However, one distinctive member of the YkuD-type transpeptidase family, LdtF (recently renamed DpaA), carries out the opposite reaction of detaching Lpp from the peptidoglycan layer. DpaA specifically hydrolyzes the amide bond between mDAP in PG and the C-terminal L-lysine of Lpp, in a reaction that is the opposite of the Lpp attachment reactions catalyzed by some of the Ldt enzymes. In this study, we report the crystal structure of DpaA, which reveals the enzyme’s ability to cleave, rather than form, the Lpp-peptidoglycan linkage. Assays with purified peptidoglycan-Lpp as the substrate and chemically synthesized compounds suggest that DpaA’s shallow L-shaped active site can only accommodate and cleave the peptidoglycan-Lpp cross-link with a constrained conformation.

However, by treating purified sDpaA with V8 protease, we were able to obtain crystals of the V8-trimmed wild-type sDpaA. Subsequently, we collected a 2.9 Å resolution data set using synchrotron radiation. sDpaA forms a pseudosymmetric dimer in the crystal structure. The final model for both chains A and B in the asymmetric unit includes residues 36-229 and 36-224, respectively. Unlike other YkuD family members, DpaA is a compact protein of a single domain composed of a single mixed five-stranded β-sheet (β1-3 and β4-5), which is flanked by four α-helices and one pair of β-strands (β6-7). Unlike other YkuD-like transpeptidases, sDpaA’s second mixed β-sheet region (Val98-Ala145) is degenerated and instead consists of five coiled strands that are connected by only a few backbone hydrogen bonds. The catalytic Cys143 residue is located in a sharp elbow turn of the coils and is surrounded by three loops (L1–3). These loops create a shallow substrate-binding groove. Our study has revealed that DpaA forms a shallow substrate-binding cleft, with the catalytic Cys143 accessible through a single entrance, similar to LD-CPases. By contrast, DpaA and CPases have a shortened L2 loop, resulting in an uncovered substrate-binding site.

>MGLLGSSSSTTPVSKEYKQQLMGSPVYIQIFKEERTLDLYVKMGEQYQLLDSYKICKYSGGLGPKQRQGDFKSPEGFYSVQRNQLKPDSRYYKAINIGFPNAYDRAHGYEGKYLMIHGDCVSIGCYAMTNQGIDEIFQFVTGALVFGQPSVQVSIYPFRMTDANMKRHKYSNFKDFWEQLKPGYDYFEQTRKPPTVSVVNGRYVVSKPLSHEVVQPQLASNYTLPEAKLEHHHHHH[2x]> PTIQPTQPTTQLPTDSPTQPTTGSFCPGPVTLCSDLESHSTEAVLGDALVDFSLKLYHAFSAMKKVETNMAFSPFSIASLLTQVLLGAGENTKTNLESILSYPKDFTCVHQALKGFTTKGVTSVSQIFHSPDLAIRDTFVNASRTLYSSSPRVLSNNSDANLELINTWVAKNTNNKISRLLDSLPSDTRLVLLNAIYLSAKWKTTFDPKKTRMEPFHFKNSVIKVPMMNSKKYPVAHFIDQTLKAKVGQLQLSHNLSLVILVPQNLKHRLEDMEQALSPSVFKAIMEKLEMSKFQPTLLTLPRIKVTTSQDMLSIMEKLEFFDFSYDLNLCGLTEDPDLQVSAMQHQTVLELTETGVEAAAASAISVARTLLVFEVQQPFLFVLWDQQHKFPVFMGRVYDPRA;> AVTAAQRIDGGAAFLGDVAIATTKASEHGINVTGRTAEVRVTGGTIRTSGNQAQGLRVGTENAPDNTAVVASVFLQNLIIETSGTGALGVSVHEPQGGGGTRLSMSGTTVRTRGDDSFALQLSGPASATLNDVALETAGQQAPAVVLWQGAQLNAQGLVVQVNGAGVSAIHAQDAGSFTLSGSDITARGLEVVGIYVQEGMQGTLTGTRVTTQGDTAPALQVEDAGTHVSMNGGALSTSGANSPAAWLLAGGSAQFRDTVLRTVGEASHGVDVAAHSEVELAHAQVRADGQGAHGLVVTRSSAMVRAGSLVESTGDGAAALLESGHLTVDGSVVHGHGAAGLEVDGESNVSLLNGARLSSDQPTAIRLIDPR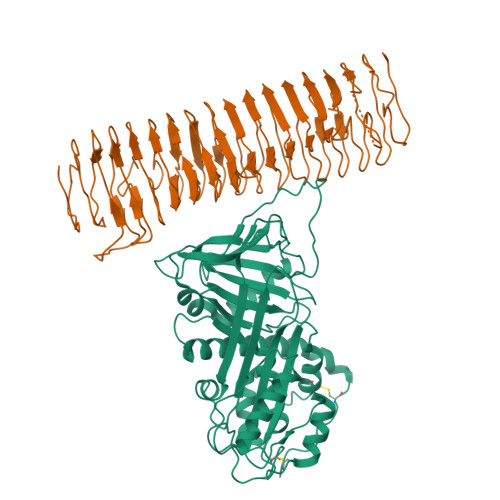SVLNLDIKDRAQLLGDIAPEAQQPDGSPEQARVRVALADGGTWAGRTDGAVHTVRLLDRGVWTVTGDSRVAEVKLEGGTLAFAPPAQPKGAFKTLVATQGISGTGTIVMNAHLPSGTADVLVAPQGFGDRQVLVVNNTDDGTESGATKVPLIEDEQGHTAFTLGNMGGRVDAGARQYELTASEAQADKARTWQLTPTNELSTTATAAVNAMAIAASQRIWQAEMDVLLRHMSGLHSIGSPGGFWARGLSQRQRLDTGYGPWQKQTVSGIELGLDRRVAGGATTAWSVGMLAGYSETRRDGGAYRAGHVHSAHVGAYVSYLNDSGSYVDGVVKYNRFRHGFDIRTTDLKRVDAKHRSHGLGALLRGGRRIDIDGGWYVEPQASVAWFHAGGSRYEASNGLRVRADGAHSWVLRAGAEAGRQMRLANGNIVEPYARLGWAQELGADNAVYTNGIRHVTRSRGGFAEARVGVGALLGKRHALYADYEYAKGARFEAPWTLQLGYRYSW> GPDSMVLLSSSWLPLNKDIEVEVVDYLPSSSVAPDLFALTLLRINDSSMKEKYDSMHEKMNAYAQIVPFDSELEIGYDGVFRDAPRSVRRVRRISATKLYLVDFGKIINYEKAKCFQLPKVFQSMPTRVSLCGLDGLTWSPV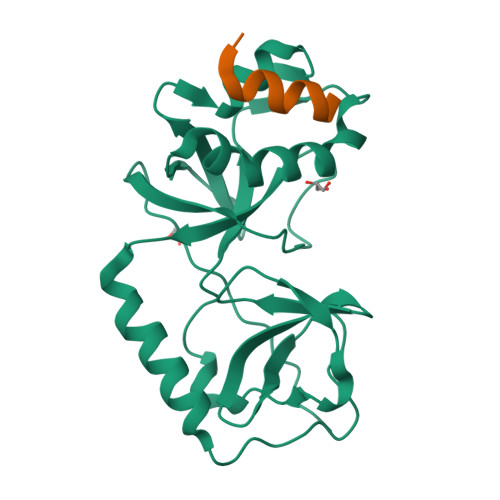AIPSFDNIREVVKKWGQMENSTLHAMACGFQGSINMINLFCGKSILADRLQRKGVCEYL;> GPDSMEVEESLLDALLGKALAGDQMNSRIEGLFEDLD> G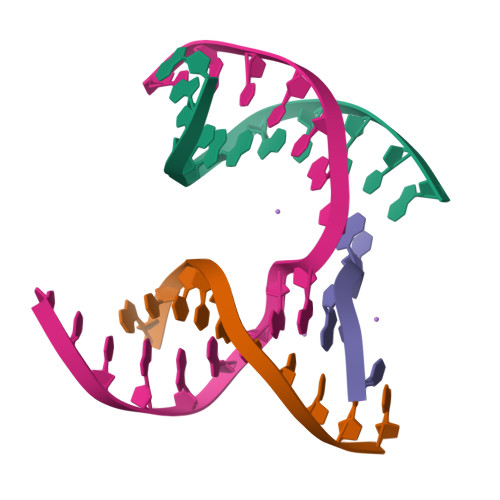AGCAGACATG;> ACTCCACTCA;> CAAGT;> TCTGAGTGGTGTCTGC> ESQPDPMPDDLHKSSEFTGTMGNMKYLYDDHYVSATKVKSVDKFLAHDLIYNISDKKLKNYDKVKTELLNEDLAKKYKDEVVDVYGSNYYVNCYFSSKDNVWWHGKTCMYGGITKHE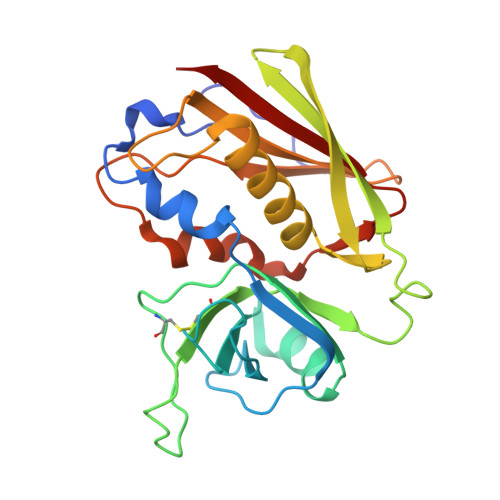GNHFDNGNLQNVLVRVYENKRNTISFEVQTDKKSVTAQELDIKARNFLINKKNLYEFNSSPYETGYIKFIENNGNTFWYDMMPAPGDKFDQSKYLMMYNDNKTVDSKSVKIEVHLTTKNG> LLQKYVTWDEHSIFVNGERL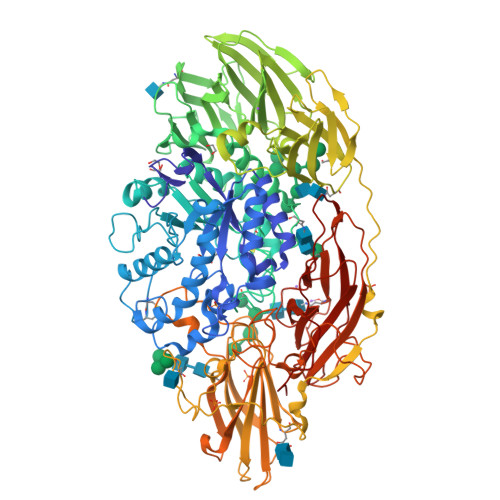MIFSGEVHPYRLPVASLYIDIFEKVKALGFNCVSFYVDWALLEGNPGHYSAEGIFDLQPFFDAAKEAGIYLLARPGPYINAEVSGGGFPGWLQRVDGILRTSDEAYLKATDNYASNIAATIAKAQITNGGPIILYQPENEYSGACCGYNGFPDGSYMQYIEDHARDAGIVVPFISNDAWAAGHNAPGTGAGAVDIYGHDSYPLGFDCANPSTWPSGNLPTYFHTSHEQQSPSTPYSLVEFQGGAFDPWGGVGFAKCAALLNHEFERVFYKNDFSFGVAFLNLYMIFGGTNWGNLGHPGGYTSYDYGSAISESRNITREKYSELKLLGNFAKVSPGYLVANPGDLSTSTYTNTADLTVTPLLGSNSSASSFFVIRHSDYSSQASVEYKLTVPTSAGNLTIPQLGGSLTLSGRDSKIHVTDYDVAGTNILYSTAEVFTWKKFNNEKVLVLYGGPGEHHEFAVSGASSSSVVEGSSSGISSKKVGKALVVAWDVSTARRIVQVGSLKVFLLDRNSAYNYWVPQVPTKGTAPGYSNQETTASSIIVKAGYLVRSAYLDGNDLHIQADFNATTPIEVVGAPSGAKNLVINGKKTQTKVDKNGIWSASVAYTAPKVQLPSLKSLKWKSVDTLPEAKNTYDDSAWTSADHAYTNNSAHSLQTPTSLFASDYGYHTGALLFRGHFTANGKEKTFFVQTKGGTAYGHSIWINETYVGSWAGTSINDNNNATYTLPTLQSGKNYVITVVIDNMGLDEDWTIGSEDMKNPRGIIQYSLSGQEASAISWKLTGNLGGENYRDTVRGPLNEGGLYAERQGFHQPQPPTQKWDSSSPFTGLTKPGIRFYSTSFDLDLPSGYDIPLYFNFGNSTSTPAAYRVQLYVNGYQYGKYVNNIGPQTSFPVPEGILNYHGTNWLALSLWAQEDNGAKLDSFELINTTPVLTSLGEVKSVNQPKYQARKGAY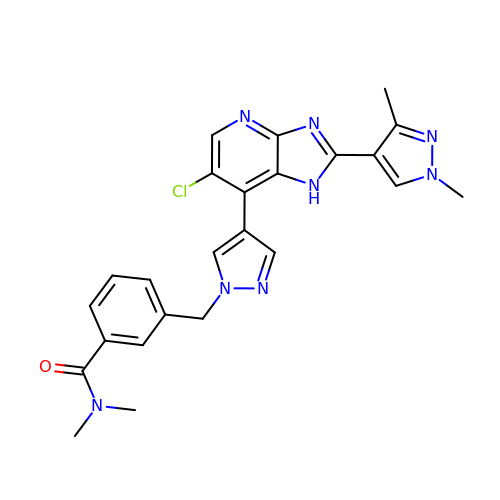3-((4-(6-chloro-2-(1,3-dimethyl-1H-pyrazol-4-yl)-3H-imidazo[4,5-b]pyridin-7-yl)-1H-pyrazol-1-yl)methyl)-N,N-dimethylbenzamide | C24 H23 Cl N8 O | SAMGYEUAKOLWAS-UHFFFAOYSA-N> MIINGTSFEELYNGLRNRGKDKKTIQLYVSPTVDAIVCYKILSMMFEKDGLLHSAVPVNNYETLSRVFKETIGHTDVHTVFFIDCAGSIDVSELLGDIENIFVYIIDSHRPFNKLNVTNTNIGLITSNEYQQFIEQETQLEKSDLLEVDDDLIGLNKSQSFNNCEYIRKMVDSDGEFYSESVGRVALAIAKKLNKVENDMYWYAAIGVCDQYISLKINAKTYVHAIQYFIDNLQLETLEITDLLQTVKTPMCVKMDCQLMLLRHWTLYDSLFHTREIASKLGIWTSRGKEKFDVLIADMGIPLSQAQQSYKTMSLEMKNKFLLKMEGYSKFYHFENLFLPSFFKKFGMDYSISAFDAAHAIGSIITNDEPDQNWQQQFWEGFKLLSSTTAEPYDFGFAKCIESNKNLVETGIILLLSGSCFNEANKYRFCSVSDELLSIRFKTPYKALQLAQFLAEASSRRYKKWLPFILAVLDAEKKTFVIVGYSSPISVKTLNYFGAKFTQTAQNMKISILQKSFDSFVTE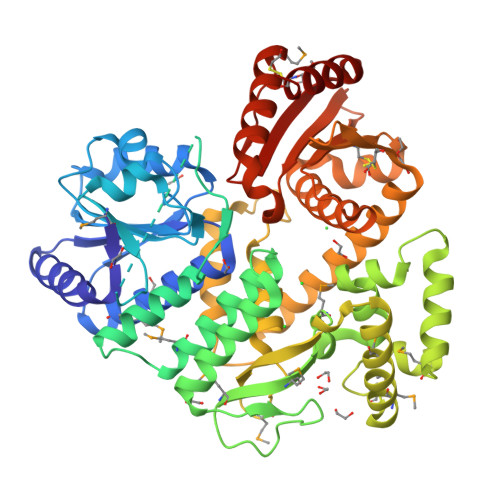IHRENLVKYKKALHKCFTSI>MHHHHHHITSLYKKAGSEFALDSSKLEAIYATSEADRDYKENAVDGDENTIWHSAYQAADKLPVSITIKLDKAYDLNQIDYLPRQNSRNGHVTEYKIETSLDNENWTEVRTGNLEVNEAGNALANRGYNPIRFNTINAQ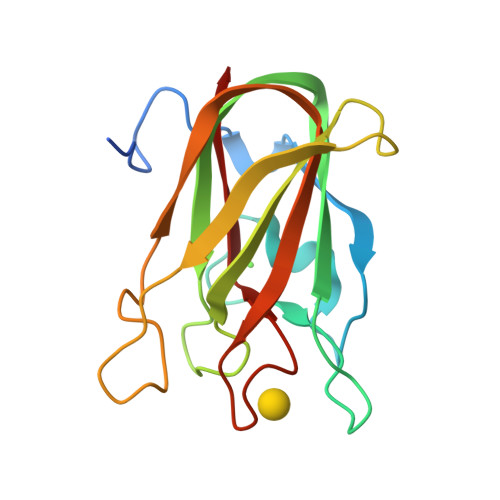YLRFTALKTLGDTNNKYASAAELVFYGK[2x]>[6x]ED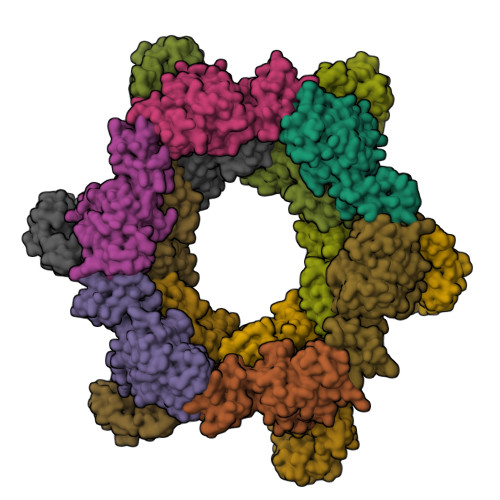PHLRNRPGKGHNYIDGMTQEDATCKPVTYAGACSSFDVLLEKGKFPLFQSYAHHRTLLEAVHDTIIAKADPPSCDLQSAHGNPCMKEKLVMKTHCPNDYQSAHYLNNDGKMASVKCPPKYELTEDCNFCRQMTGASLKKGSYPLQDLFCQSSEDDGSKLKTKMKGVCEVGVQALKKCDGQLSTAHEVVPFAVFKNSKKVYLDKLDLKTEENLLPDSFVCFEHKGQYKGKLDSGQTKRELKSFDISQCPKIGGHGSKKCTGDAAFCSAYECTAQYANAYCSHANGSGIVQIQVSGVWKKPLCVGYERVVVKRELS;>DPGCSELIQASSRITTCSTEGVNTKCRLSGTALIRAGSVGAEACLMLKGVKEDQTKFLKIKTVSSELSCREGQSYWTGSFSPKCLSSRRCHLVGECHVNRCLSWRDNETSAEFSFVGESTTMRENKCFEQCGGWGCGCFNVNPSCLFVHTYLQSVRKEALRVFNCIDWVHKLTLEITDFDGSVSTIDLGASSSRFTNWGSVSLSLDAEGISGSNSFSFIESPGKGYAIVDEPFSEIPRQGFLGEIRCNSESSVLSAHESCLRAPNLISYKPMIDQLECTTNLIDPFVVFERGSLPQTRNDKTFAASKGNRGVQAFSKGSVQADLTLMFDNFEVDFVGAAVSCDAAFLNLTGCYSCNAGARVCLSITSTGTGSLSAHNKDGSLHIVLPSENGTKDQCQILHFTVPEVEEEFMYSCDGDERPLLVKGTLIAID[6x]>[10x]MSEGRIPLIGEK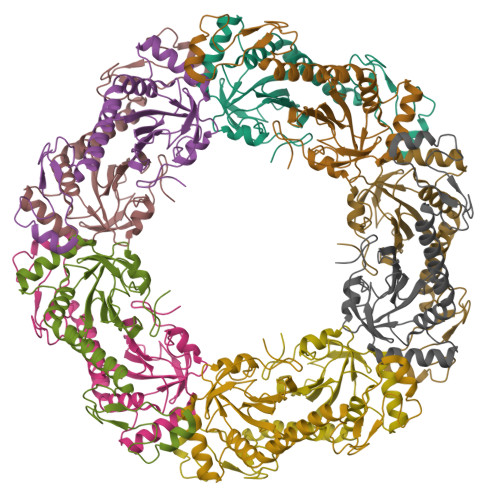FPEMEVITTHGKIKLPDDYKGRWFVLFSHPGDFTPVCTTEFYSFSKKYEEFKKLNTELIGLSVDSNISHIEWVMWIEKNLKVEVPFPIIADPMGNVAKRLGMIHAESSTATVRAVFIIDDKGTVRLILYYPMEIGRNIDEILRAIRALQLVDKAGVVTPANWPNNELIGDKVINPAPRTIKDAKMRLGQPFDWWFTYKEVKTT> GUUACUCACCUCUUCGGAGAAAACGGUCCGAGCGUGGUUCGCCACUAAAAUACCGUUUUGGCCUGAAUGUGUCUGGUCCUUCCGCAGCCGUUUGAUGAGUUCGCUCAUCAUAGCGGGCUUACCAAACAGUUCGCUG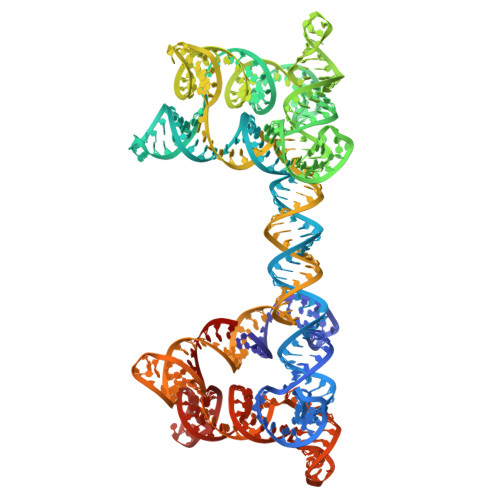CCACCGUGCGGAAGCAGUUUCGACUGAUAGAUCACGGUGGGACUAUUCGUAGUCUUUGGUGAGCUCGUUACGUUUCUUCGGAAACGAACGGCUGAUCUAUGACCAGAUGUAUUCAGGCCGUGAGUAACGUCGCCGUACAUCUUCGGAUGUAGCGUCCCUAUUUUACAAACUUCGGUUUGGCUCGGAGGGACGCAGCAGGGUUCGCCCUGCUCGGCGAC>MSDDFLWFEGIAFPTMGFRSETLRKVRDEFVIRDEDVIILTYPKSGTNWLAEILCLMHSKGDAKWIQSVPIWERSPWVESEIGYTALSETESPRLFSSHLPIQLFPKSFFSSKAKVIYLMRNPRDVLVSGYFFWKNMKFIKKPKSWEEYFEWFCQGTVLYGSWFDHIHGWMPMREEKNFLLLSYEELKQDTGRTIEKICQFLGKTLEPEELNLILKNSSFQSMKENKMSNYSLLSVDY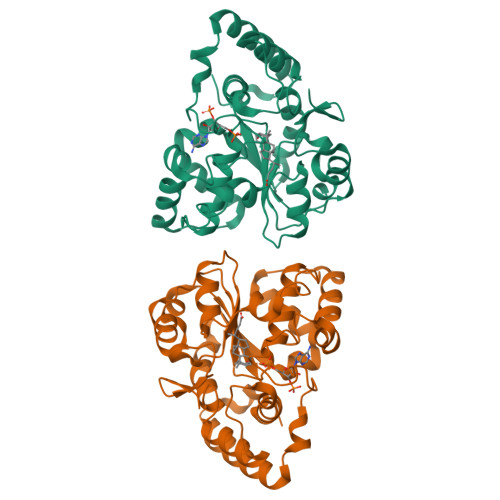VVDKAQLLRKGVSGDWKNHFTVAQAEDFDKLFQEKMADLPRELFPWE[4x]> MHHHHHHSSGRENLYFQGVWKSYLYQLQQEAPHPRRITCTCEVENRPKYYGREFHGMISREAADQLLIVAEGSYLIRESQRQPGTYTLALRFGSQTRNFRLYYDGKHFVGEKRFESIHDLVTDGLITLYIETKAAEYIAKMTINPIYEHVGYTTLNREPAYKKHMPVLKETHDERDSTGQDGVSEKRLTSLVRRATLKENEQIPKYEKIHNFKVHTFRGPHWCEYCANFMWGLIAQGVKCADCGLNVHKQCSKMVPNDCKPDLKHVKKVYSCDLTTLVKAHTTKRPMVVDMCIREIESRGLNSEGLYRVSGFSDLIEDVKMAFDRDGEKADI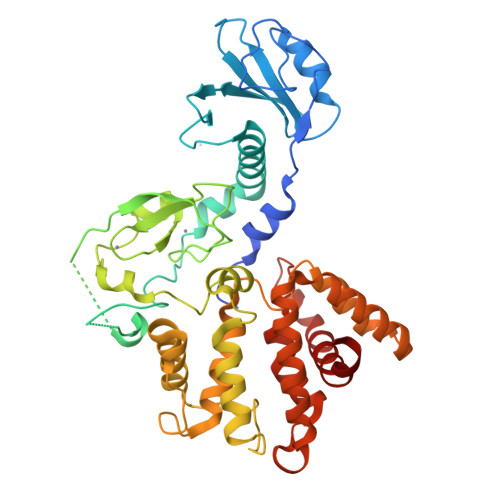SVNMYEDINIITGALKLYFRDLPIPLITYDAYPKFIESAKIMDPDEQLETLHEALKLLPPAHCETLRYLMAHLKRVTLHEKENLMNAENLGIVFGPTLMRSPELDAMAALNDIRYQRLVVELLIKNEDILF Clopidogrel | C16 H16 Cl N O2 S | 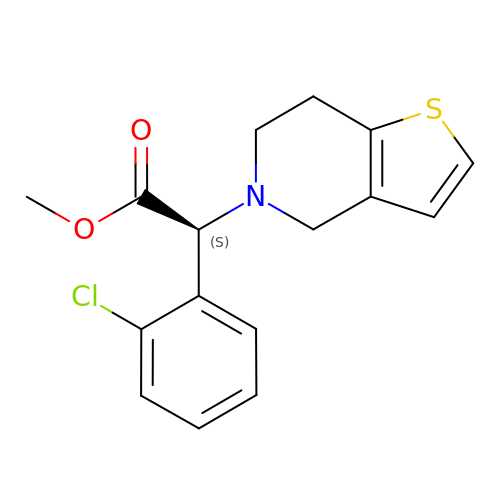GKTWGGQPFAXNFI-HNNXBMFYSA-N>[4x]MNVTVDQSTLAGATRGIVRGGETLKEHRDRLMAATKATGRYAGLKTLELREREPILYNKLFSRLRAGVVDARETAKKIAASPIVEQEGELCFTLYNAAGDSLLTSTGIIIHVGTMGAAIKYMIENNWEANPGVHDKDIFCNNDSLIGNVHPCDIHTIVPIFWEGELIGWVGGVTHVIDTGAVGPGSMATGQVQRFGDGYSITCRKVGANDTLFRDWLHESQRMVRTTRYWMLDERTRIAGCHMIRKLVEEVVAEEGIEAYWKFAYEAVEHGRLGLQARIKAMTIPGTYRQVGFVDVPYAHEDVRVPSDFAKLDTIMHAPCEMTIRRDGTWRLDFEGSSRWGWHTYNAHQVSFTSGIWVMMTQTLIPSEMINDGAAYGTEFRLPKGTWMNPDDRRVAFSYSWHFLVSAWTALWRGLSRSYFGRGYLEEVNAGNANTSNWLQGGGFNQYDEIHAVNSFECAANGTGATAVQDGLSHAAAIWNPEGDMGDMEIWELAEPLVYLGRQIKASSGGSGKYRGGCGFESLRMVWNAKDWTMFFMGNGHISSDWGLMGGYPAASGYRFAAHKTNLKELIASGAEIPLGGDTDPENPTWDAMLPDAQIKRDKQAITTEEMFSDYDLYLNYMRGGPGFGDPLDREPQAVADDINGGYVLERFAGEVYGVVVRKGADGQYGVDETATAAARAQIRKDRLAKSVPVSEWMKGEREKILAKDAGTQVRQMFAASFKLGPRFEKDFRTFWDLPDSWTLPEEEIGVPTYGSRYSMDISELPDVHTVQFVEE;>MNVPVGHLRNVQVLGIDAGGTMTDTFFVDQDGDFVVGKAQSTPQNEALGLIASSEDGLANWGMSLHEALAQLQTGVYSGTAMLNRVVQRKGLKCGLIVNRGMEDFHRMGRAVQSHLGYAYEDRIHLNTHRYDPP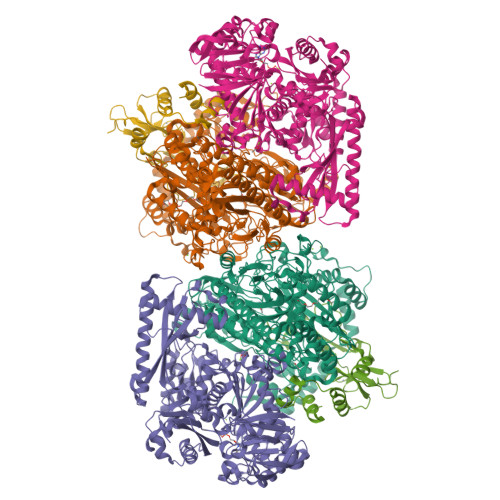LVPRHLTRGVVERTDMMGTQVIPLREDTARDAARDLIAADAEGIVISLLHSYKNPVNERRVRDIVLEEVEKSGKKIPVFASADYYPVRKETHRTNTTILEGYAAEPSRQTLSKISNAFKERGTKFDFRVMATHGGTISWKAKELARTIVSGPIGGVIGAKYLGEVLGYKNIACSDIGGTSFDVALITQGEMTIKNDPDMARLVLSLPLVAMDSVGAGAGSFIRLDPYTRAIKLGPDSAGYRVGVCWKESGIETVTISDCHMVLGYLNPDNFLGGAVKLDRQRSVDAIKAQIADPLGLSVEDAAAGVIELLDSDLRDYLRSMISGKGYSPASFVCFSYGGAGPVHTYGYTEGLGFEDVIVPAWAAGFSAFGCAAADFEYRYDKSLDINMPTETPDTDKEKAAATLQAAWEELTKNVLEEFKLNGYSADQVTLQPGYRMQYRGQLNDLEIESPLAQAHTAADWDQLTDAFNATYGRVYAASARSPELGYSVTGAIMRGMVPIPKPKIPKEPEEGETPPESAKIGTRKFYRKKRWVDAQLYHMESLRPGNRVMGPAVIESDATTFVVPDGFETWLDGHRLFHLREV[4x];>MAYTRSKIVDLVDGKIDPDTLHQMLSTPKDPERFVTYVEILQERMPWDDKIILPLGPKLFIVQQKVSKKWTVRCECGHDFCDWKDNWKLHARVHVRDTPQKMEEIYPRLMAPTPSWQVIREYFCPECGTLHDVEAPTPWYPVIHDFSPDIEGFYQEWLGLPVPERADA[4x]>MTSTGRFTLPSEENFAEKTKELAELWGADAIRNSDGTHLDEAVLALGKKIYNAYFPTRAHNEWITLHMDETPQVYLLTDRILAESDTVDIPLMESFFAEQLKPNRDADPHKYWEVVDRTTGEVVDSANWTLDADEDTVHVSGVAAWHEYTVSFLAYIIWDPVEMYNHLTNDWGDKEHEIPFDIYHPATRKFVFDTFEQWLKDSPQTDVVRFTTFFYQFTLLFDEKRREKVVDWFGCACTVSPRALDDFEAKYGYRLRPEDFVDGGAYNSAWRVPRKAQRDWIDFLSGFVRENVKQLADMSHAAGKEAMMFLGDQWIGTEPYKDGFDELGLDAVVGSIGDGTTTRMIADIPGVKYTEGRFLPYFFPDTFYEGNDPSIEGLDNWRKARRAILRSPISRMGYGGYLSLAAKFPKFVDTVTHIANEFRDIHDRTGGVAAEGELNVAILNSWGKMRSWMAFTVAHALPNKQTYSYYGILESLSGMRVNVRFISFDDVLAHGIDSDIDVIINGGPVDTAFTGGDVWTNPKLVETVRAWVRGGGAFVGVGEPSSAPRFQTGRFFQLADVIGVDEERYQTLSVDKYFPPVVPDHFITADVPVDPAAREAWEQAGYRIPLSGCGGGQSIKPLGGIDFGEPVLNTYPVNENVTLLRADGGQVQLATNDYGKGRGVYISGLPYSAANAR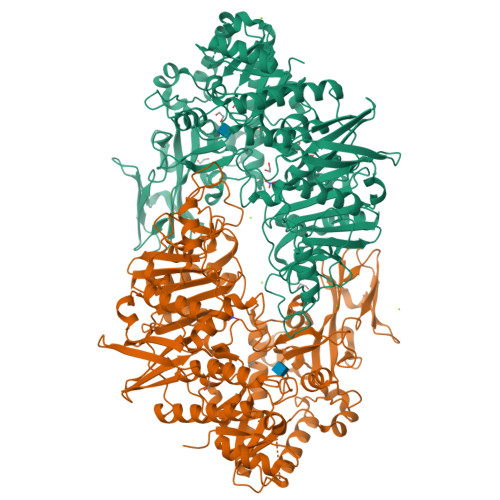LLERVLFYASHNEDKYAAWSSSNPECEVAHFPEQGLYCVINNTDQPQKTTVTLADGTTEDFDLPDSGIAWREALEHHHHHH[2x]> GPHMSEAYFRVESGALGPEENFLSLDDILMSHEKLPVRTETAMPRLGAFFLERSAGAETDNAVPQGSKLELPLWLAKGLFDNKRRILSVELPKIYQEGWRTVFSADPNVVDLHKMGPHFYGFGSQLLHFDSPENADISQSLLQTFIGRFRRIMDSSQNAYNEDTSALVARLDEMERGLFQTGQKGLNDFQCWEKGQASQITASNLV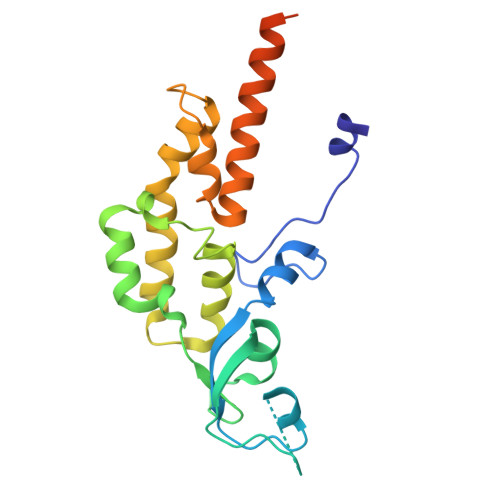QNYKKRKFTDMED> DQTAPGTASRPILTASESNYFTTATYLQGWSPPSISTSKADYTVGNGYNTIQAAVNAAINAGGTTRKYIKINAGTYQEVVYIPNTKVPLTIYGGGSSPSDTLITLNMPAQTTPSAYKSLVGSLFNSADPAYSMYNSCASKSGTIGTSCSTVFWVKAPAVQIVNLSIENSAKNTGDQQAVALQTNSDQIQIHNARLLGHQDTLYAGSGSSSVERSYYTNTYIEGDIDFVFGGGSAIFESCTFYVKADRRSDTAVVFAPDTDPHKMYGYFVYKSTITGDSAWSSSKKAYLGRAWDSGVSSSSAYVPGTSPNGQLIIKE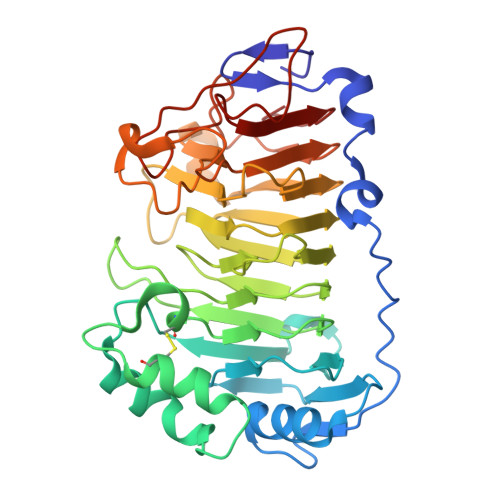STIDGIINTSGPWTTATSGRTYSGNNANSRDLNNDNYNRFWEYNNSGNGA>[4x]SNAYKMESRIKDISLAEFGLQDMEIAKTDMMGLVELQRKYRDSKPLKGARITGSLHLTIETSVLVETLYELGAEIRWCSCNIYSTQDHAAAALVKKNIATVFAWKNETIEDYWVCLNDAMTWRNPNDKDKICGPNLIVDDGGDATLILHEGVKAEIEYEKYNKIPEYLETELDENGKQLSMDLKCMYKVLKMELLKNPFRWRGMLKDLYGVSEET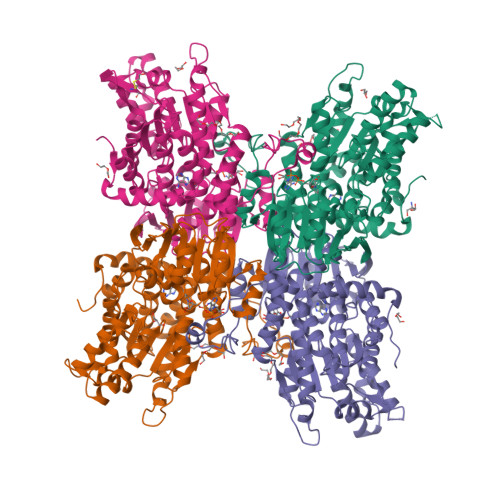TTGVLRLKIMESEGKLLLPAINVNDSVTKSKFDNTYGCRQSLLHGLFNGCIQMLAGKKIVVLGYGEVGKGCAQGLSGVGARVIVTEIDPICALQASMEGYQVSVLEDVVSEADIFITATGNKDVITVEHMRKMKENAYIANIGHFDDEIDVYGLENYPGIKVIEVKQNVHKFTFPDTQKSVILLCKGRLVNLGCATGHPPLVMSMSFTNQVLAQMDLWKSRELVDRSKNTRFFVKKLSKELDEYVARLHLDVLGIKLTKLTETQAKYINVSINGPYKSEDYRY>[2x]NVLTVYSPYQSNLIRPILNEFEKQEHVKIEIKHGSTQVLLSNLHNEDFSERGDVFMGGVLSETIDHPEDFVPYQDTSVTQQLEDYRSNNKYVTSFLLMPTVIVVNSDLQGDIKIRGYQDLLQPILKGKIA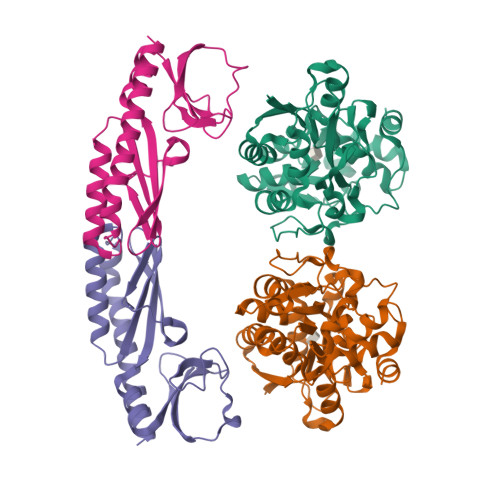YSNPNTTTTGYQHMRAIYSMHHRVSDVHQFQNHAMQLSKTSKVIEDVAKGKYYAGLSYEQDARTWKNKGYPVSIVYPIEGTMLNVDGIALVKNAHPHPKRKKLVQYLTSRSVQQRLVAEFDAKSIRKDVSEQSDQSIENLKNIPLIPKSKLPDIPHHKFLEMIQ;>[2x]TIHQHVDESQSSLHHTEKQIQTFITQHNNSFQELDLTNHHDVTATKRELLKLIHQQPATLYYELSGPNQFITNNYEHLNTKNMYLFSTHQLKFKNSTYMLKIYMANTPRLSEIKKDNRQFALIVDQYDNILYANDDRFTIGEKYRPQQFGFMNESVKLNHADHRLIIYKDI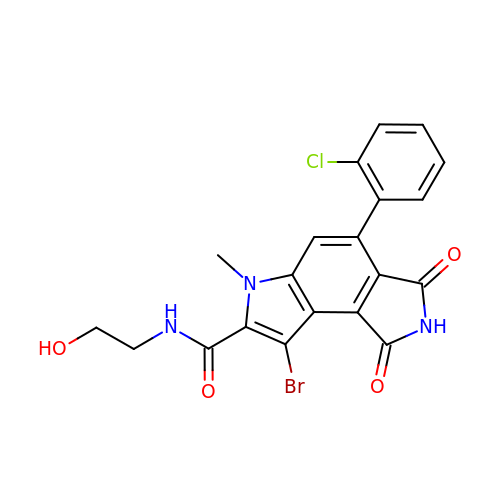8-bromo-4-(2-chlorophenyl)-N-(2-hydroxyethyl)-6-methyl-1,3-dioxo-1,2,3,6-tetrahydropyrrolo[3,4-e]indole-7-carboxamide | C20 H15 Br Cl N3 O4 | XUAHLMVOYLUYSB-UHFFFAOYSA-N>[2x]SNAMNIQSELEFKFAHYLINNAVE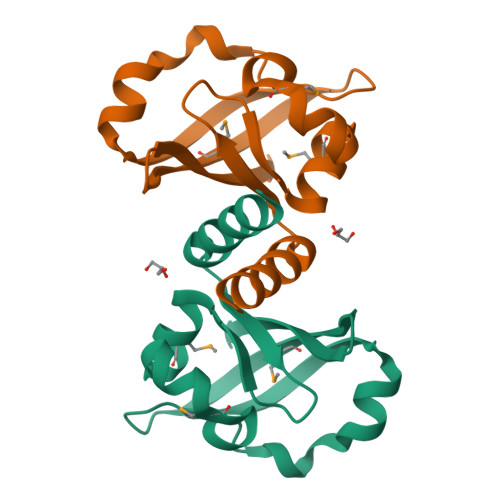ASFCLGDNWQFLYVNDATCRMTEYSREQLLSMNLQDIDVDFALHDWEEIRQKNNYTFKTRYRSQSGRIFLVEMSLTFLEDQERRFSCVFVREKS> MIRGSSALKSLTSRRLYSTGVKYTTLSNGVTVATETNPAAKTSSVGLFFGAGSRSEHSHSNGISALTTNVLASQSAKGSLLTAKNDREFNGIIAQTTNDNITEAGKLIASIASNAVDIVEKTDLTKHKQYLSAQASAVEADPKSKVLSHLYSSAFQGYSLALPTLGTTESVENLENQDSLRHLAKHLVNNNTVIAASGNFDHDKLADAIEANLKIAEGVKPEIKPASFLGSE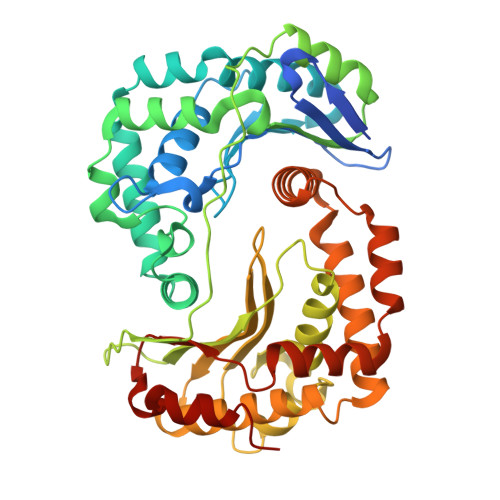VRMRDDTLPKAYISIAVHGEGLNSPNYYLAKVAAAIYGDFYLHSTIAKFTSPKLASIVQEYNIVESYNHYSKSFSDTGIWGYYAEIADKFTVDDFTHFSLKEWNRLSISISEAEVARAKAQVKTALAKELANSFAVTSDIAEKVLLVGHRQSLREAFEKIDAIKVNDVKEWGKSKVWDRDIVISGTGLIEDLLDYNRNRNEMAMMRW>DYKDDDDKAAAGDATFPKAMDNVTVRQGESATLRCTIDNRVTRVAWLNRSTILYAGNDKWCLDPRVVLLSNTQTQYSIEIQNVDVYDEGPYTCSVQTDNHPKTSRVHLIVQVSPKIVEISSDISINEGNNISLTCIATGRPEPTVTWRHISPKAVGFVSEDEYLEIQGITREQSGDYECSASNDVAAPVVRRVKVTVN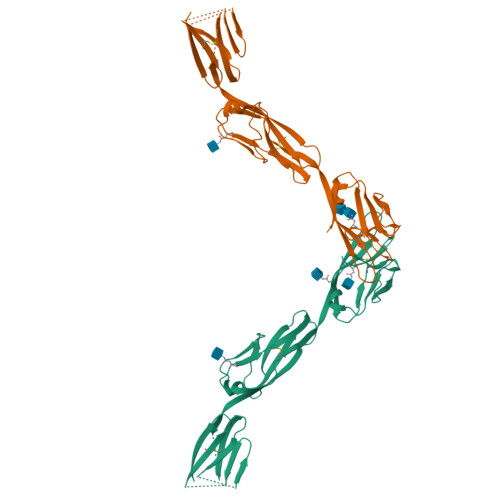YPPYISEAKGTGVPVGQKGTLQCEASAVPSAEFQWYKDDKRLIEGKKGVKVENRPFLSKLIFFNVSEHDYGNYTCVASNKLGHTNASIMLFGPGAVSEVSNGLEVLFQ[2x]> KLL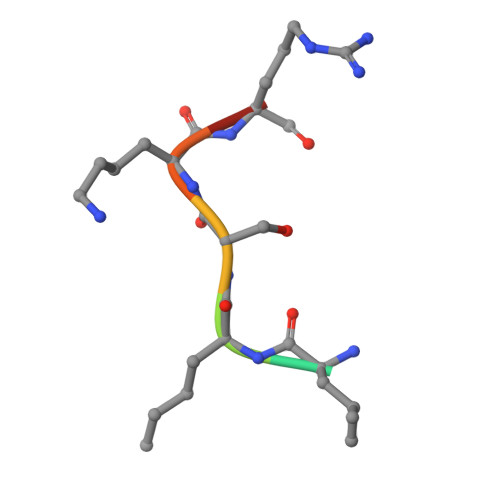SKRG calcitroic acid | C23 H34 O4 | 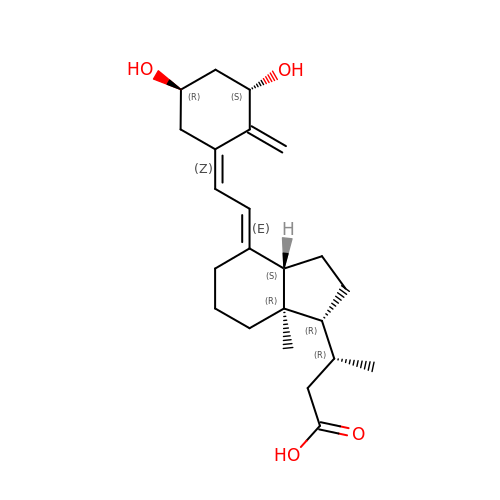MBLYZRMZFUWLOZ-ZTIKAOTBSA-N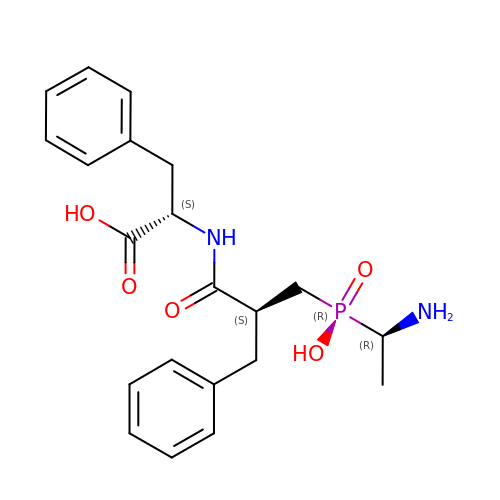N-{(2S)-3-[(1R)-1-aminoethyl](hydroxy)phosphoryl-2-benzylpropanoyl}-L-phenylalanine | C21 H27 N2 O5 P | MMWNOZXGYRPSCJ-LZQZEXGQSA-N>MGETVVRDAVTIGKPAEQLYAVWRDLPGLPLLMTHLRSVEVLDDKRSRWTVEAPAPLGTVSWEAELTADEPGKRIAWRSLPGARIENSGEVLFRPAPGARGTEVVVRLTYRPPGGSAGAVIARMFNQEPSQQLRDDLMRFKRE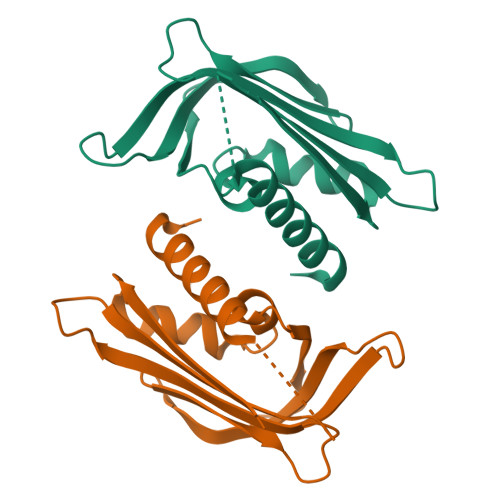QELGLEHHHHHH[2x]> QGPAMAGNLYGRDGAAIGSLQKLRFFPLAVAGGQGARLVEEDGRELIDLSGAWGAASLGYGHPAIIEAVSRAAANPAGASILSASNAPAVALAERLTASFPGRGTHKVWFGHSGSDANEAAYRAITRATGRTGVIAFIGAYHGCTVGSMAFSGHSVQADAAKADGLILLP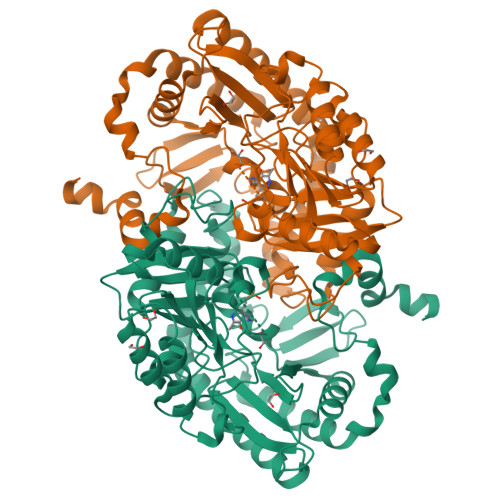YPDPYRPYQDDPTGDAVLALLKERLAAVPAGSIAAAFIEPIQSDGGLIVPPDGFLRKFADICRAHGISVVCDEVKVGLARSGRLHCFEHEGFVPDILVLGKGLGGGLPLSAVIAPAEILDCASAFAMQTLHGNPVCAAAGLAVLETIEAENLTTAAERKGKLLREGLARLAERHELIGDIRGRGLACGVELVRNRQSREPARAETAKLIYRAYELGLVLYYVGMNGNVLEMTPPLTMTEDEVRHAVNLLDQAFTELSTVSDTLVSQFAGW>ADEKPDVIDDDIQDEFPDYGFNCEFGWGSHKTFCHWEHDNHVQLKWSVLTSKTGPIQDHTGDGNFIYSQADENQKGKVARLVSPVVYSQNSAHCMTFWYHMSGSHVGTLRVKLRYQKPEEYDQLVWMAIGHQGDHWKEGRVLLHKSLKLYQVIFEG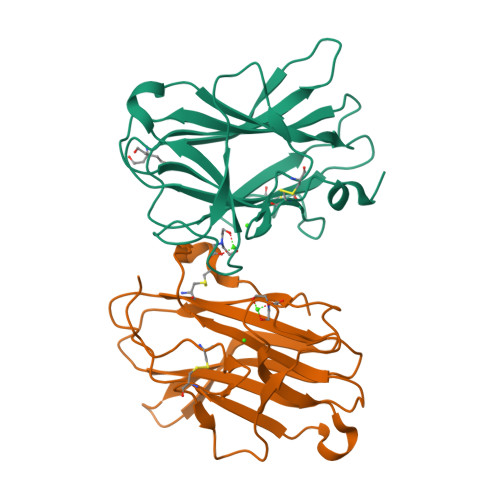EIGKGNLGGIAVDDISINNHISQEDCAKPAHHHHHH[2x]> DLPDVQELITQVRSEKCSLQAAAILDANDAHQTETSSSQVKDNKPLVERFETFCLDPSLVTKQANLVHFPPGFQPIPCKPLFFDLAL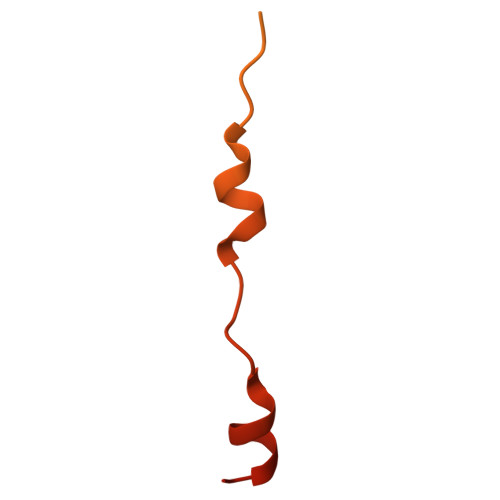NHVAFPPLEDKLAAATKSG>GTSMETFDPTELPELLKLYYRRLFPYSQYYRWLNYGGVIKNYFQHREFSFTLKDDIYIRYQSFNNQSDLEKEMQKMNPYKIDIGAVYSHRPNQHNTVKLGAFQAQEKELVFDIDMTDYDDVRRCCSSADICPKCWTLMTMAIRIIDRALKEDFGFKHRLWVYSGRRGVHCWVCDESVRKLSSAVRSGIVEYLSLVKGGQDVKKKVHLSEKIHPFIRKSINIIKKYFEEYALVNQDILENKESWDKILALVPETIHDELQQSFQKSHNSLQRWEHLKKVASRYQNNIKNDKYGPWLEWEIMLQYCFPRLDINVSKGINHLLKSPFSVHPKTGRISVPIDLQKVDQFDPFTVPTISFICRELDAISTNEEEKEENEAESDVKHRTRDYKKTSLA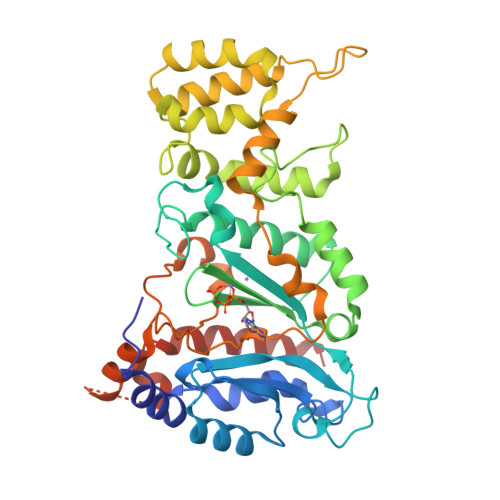PYVKVFEHFLENLDKSRK[2x]>[2x]GSRRASVGSHRFKVYNYMSPTFCDHCGSLLWGLVKQGL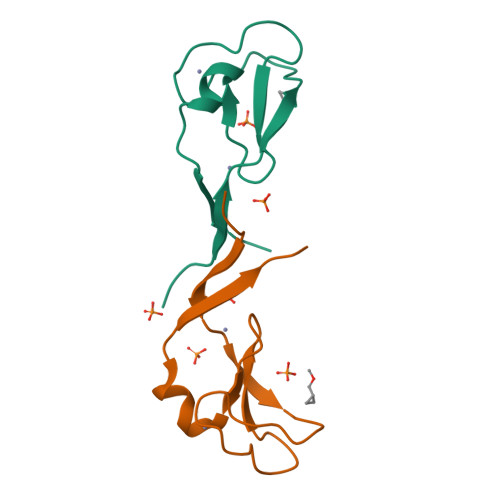KCEDCGMNVHHKCREKVANLCEFIVTD>MNHKVHMMSQPKPILYYDERSPPVRSCLMLIKLLDIDVELRFVNLFKGEQFQKDFLALNPQHSVPTLVHGDLVLTDSHAILIHLAEKFDEGGSLWPQEHAERMKVLNLLLFECSFLFRRASDFMSAIVRQGFANVDVAHHERKLTEAYIIMERYLENSDFMAGPQLTLADLSIVTTLSTVNLMFPLSQFPRLRRWFTAMQQLDAYEANCSGLEKLRQTMESVGSFQFPSSSAVVTEKVE[2x]

Here, we report the first crystal structure of an ecdysteroidogenic regulator encoded by the Halloween gene, noppera-bo (nobo). nobo encodes a member of the epsilon class of cytosolic GSH S-transferases (GST, EC 2.5.1.18; hereafter GSTEs). DmNobo forms a polypeptide homodimer with a canonical GST fold, which has a well-conserved GSH-binding site (G-site) and a hydrophobic substrate-binding pocket (H-site) adjacent to the G-site. Consistent with the requirement of GSH for GST function, a defect in GSH biosynthesis in D. melanogaster also leads to larval lethality, which is partly rescued by the administration of 20E or cholesterol. These data indicate that the nobo family of GSTs is essential for ecdysteroid biosynthesis by regulating cholesterol trafficking and/or metabolism. In general, GSTs catalyze various reactions with an activated glutathione (GSH) molecule in the following three ways: GSH conjugation to a substrate, reduction of a substrate using GSH, and isomerization.

The importance of the Asp-113–EST hydrogen bond for EST binding was biochemically examined with a recombinant mutated DmNobo protein carrying D113A amino acid substitution (DmNobo D113A). DmNobo D113A lacks the sidechain carboxyl group at position 113 and therefore cannot form a hydrogen bond with EST. The crystal structure of the DmNobo D113A did not show significant structural differences compared with the WT DmNobo (DmNobo WT) protein. In the absence of EST, both DmNobo WT and DmNobo D113A showed GSH conjugation activity although the activity of DmNobo D113A decreased by approximately half of DmNobo WT. In the presence of EST, as expected from the EST-binding to the H-site, the enzymatic activity of DmNobo WT was inhibited with an IC50 value of ∼2.3 μm. In contrast, the enzymatic activity of DmNobo D113A was not inhibited by EST, even at a concentration of 25 μm. In contrast, it was barely possible to determine the Kd value between DmNobo D113A and EST because of a weak interaction, which was consistent with crystal structure analysis. These results suggest that Asp-113 is critical for interaction with EST.> MAGLNEILLPEVHLNSPIVRYKLFYYILHGQLPNDLEPDDLGPLANQNWKAIRAEESQVHARLKQIRVELIARIPSLRWTRSQREIAILIWPRILPILQAYDLRQSMQLPTVWEKLTQSTVNLISDGLERVVLHISNQLTGKPNLFTRSRAGQDTKDYSIPSTRELSQIWFNNEWSGSVKTWLMIKYRMRQLITNQKTGELTDLVTIVDTRSTLCIITPELVALYSSEHKALTYLTFEMVLMVTDMLEGRLNVSSLCTASHYLSPLKKRIEVLLTLVDDLALLMGDKVYGIVSSLESFVYAQLQYGDPVIDIKGTFYGFICNEILDLLTEDNIFTEEEANKVLLDLTSQFDNLSPDLTAELLCIMRLWGHPTLTASQAASKVRESMCAPKVLDFQTIMKTLAFFHAILINGYRRSHNGIWPPTTLHGNAPKSLIEMRHDNSELKYEYVLKNWKSISMLRIHKCFDASPDEDLSIFMKDKAISCPRQDWMGVFRRSLIKQRYRDANRPLPQPFNRRLLLNFLEDDRFDPIKELEYVTSGEYLRDPEFCASYSLKEKEIKATGRIFAKMTKRMRSCQVIAESLLANHAGKLMRENGVVLDQLKLTKSLLTMNQIGIISEHSRRSTADNMTLAHSGSNKHRINNSQFKKNKDNKHEMPDDGFEIAACFLTTDLTKYCLNWRYQVIIPFARTLNSMYGIPHLFEWIHLRLMRSTLYVGDPFNPPSDPTQLDLDTALNDDIFIVSPRGGIEGLCQKLWTMISISTIILSATEANTRVMSMVQGDNQAIAITTRVVRSLSHSEKKEQAYKASKLFFERLRANNHGIGHHLKEQETILSSDFFIYSKRVFYKGRILTQALKNVSKMCLTADILGDCSQASCSNLATTVMRLTENGVEKDLCYFLNAFMTIRQLCYDLVFPQTKSLSQDITNAYLNHPILISRLCLLPSQLGGLNFLSCSRLFNRNIGDPLVSAIADVKRLIKAGCLDIWVLYNILGRRPGKGKWSTLAADPYTLNIDYLVPSTTFLKKHAQYTLMERSVNPMLRGVFSENAAEEEEELAQYLLDREVVMPRVAHVILAQSSCGRRKQIQGYLDSTRTIIRYSLEVRPLSAKKLNTVIEYNLLYLSYNLEIIEKPNIVQPFLNAINVDTCSIDIARSLRKLSWATLLNGRPIEGLETPDPIELVHGCLIIGSDECEHCSSGDDKFTWFFLPKGIRLDDDPASNPPIRVPYIGSKTDERRVASMAYIKGASVSLKSALRLAGVYIWAFGDTEESWQDAYELASTRVNLTLEQLQSLTPLPTSANLVHRLDDGTTQLKFTPASSYAFSSFVHISNDCQILEIDDQVTDSNLIYQQVMITGLALIETWNNPPINFSVYETTLHLHTGSSCCIRPVESCVVNPPLLPVPLINVPQMNKFVYDPEPLSLLEMEKIEDIAYQTRIGGLDQIPLLEKIPLLAHLTAKQMVNSITGLDEATSIMNDAVVQADYTSNWISECCYTYIDSVFVYSGWALLLELSYQMYYLRIQGIQGILDYVYMTLRRIPGMAITGISSTISHPRILRRCINLDVIAPINSPHIASLDYTKLSIDAVMWGTKQVLTNISQGIDYEIVVPSESQLTLSDRVLNLVARKLSLLAIIWANYNYPPKVKGMSPEDKCQALTTHLLQTVEYVEYIQIEKTNIRRMIIEPKLTAYPSNLFYLSRKLLNAIRDSEEGQFLIASYYNSFGYLEPILMESKIFNLSSSESASLTEFDFILNLELSDASLEKYSLPSLLMTAENMDNPFPQPPLHHVLRPLGLSSTSWYKTISVLNYISHMKISDGAHLYLAEGSGASMSLIETFLPGETIWYNSLFNSGENPPQRNFAPLPTQFIESVPYRLIQAGIAAGNGIVQSFYPLWNGNSDITDLSTKTSVEYIIHKVGADTCALVHVDLEGVPGSMNSMLERAQVHALLITVTVLKPGGLLILKASWEPFNRFSFLLTVLWQFFSTIRILRSSYSDPNNHEVYIIATLAVDPTTSSFTTALNRARTLNEQGFSLIPPELVSEYWRKRVEQGQIIQDCIDKVISECVRDQYLADNNIILQAGGTPSTRKWLDLPDYSSFNELQSEMARLITIHLKEVIEILKGQASDHDTLLFTSYNVGPLGKINTILRLIVERILMYTVRNWCILPTQTRLTLRQSIELGEFRLRDVITPMEILKLSPNRKYLKSALNQSTFNHLMGETSDILLNRAYQKRIWKAIGCVIYCFGLLTPDVEGSERIDVDNDIPDYDIHGDII;>MDQFIKQDETGDLIETGMNVANHFLSTPIQGTNSLSKASILPGVAPVLIGNPEQKNIQHPTASHQGSKTKGRGSGVRSIIVSPSEAGNGGTQIPEPLFAQTGQGGIVTTVYQDPTIQPTGSYRSVELAKIGKERMINRFVEKPRTSTPVTEFKRGGPGAAAQGQTIQEEGIDGNGASAGSKERSGSLSGATLYAHLSLPQQDSTPANVGIAPQSAISANEIMDLLRGMDARLQHLEQKVDKVLAQGSMVTQIKNELSTVKTTLATIEGMMATVKIMDPGNPTGVPVDELRRSFSDHVTIVSGPGDVSFSSSEKPTLYLDELARPVSKPRPAKQTKSQPVKDLAGQKVMITKMITDCVANPQMKQAFEQRLAKASTEDALNDIKRDIIRSAI[4x]

L and P function as the RNA polymerase complex, responsible for replicating and transcribing the viral genome. To catalyze the RNA synthesis in both replication and transcription, L sequentially consists of five domains: the RNA-dependent RNA polymerase domain (RdRp), polyribonucleotidyl transferase domain (PRNTase), connector domain (CD), methyltransferase domain (MTase), and C-terminal domain (CTD). P harbors an oligomerization domain (POD) for self-oligomerization, and the oligomeric P attaches to RdRp of L, tethering the polymerase to NC to extract the RNA strand for both replication and transcription. Here, we resolved two L–P complex conformations from the mumps virus (MuV), a typical member of nsNSVs, via cryogenic-electron microscopy.

The other conformation has CD-MTase-CTD averaged out due to the structural flexibility, with its RNA tunnel inaccessible to MTase, unfavorable for genome transcription. Following the same strategy, Lbody–P was determined at the resolution of 3.01 Å, and only RdRp and PRNTase are visible in L. The missing of appendage in Lbody–P indicates the structural flexibility in MuV L–P, as in other nsNSVs. MuV Lbody–P owns a flexible appendage, and its RNA tunnel is inaccessible to MTase-CTD, which is unfavorable for transcription. However, the RNA cavity formed by RdRp and PRNTase domains is available, with the potential capability for genome replication. MuV Lbody–P takes an appendage-free conformation but still owns an exposed RNA cavity formed by RdRp and PRNTase domains with the potential to another replication state for RNA synthesis. Models in (c, e) are the composite atomic models of MuV Lintegral–P and Lbody–P via rigid body docking of individual models into their respective composite cryo-EM maps, which are B-factor sharpened. In both conformations, parallel P tetramers are revealed around MuV L, which, together with structures of other nsNSVs, demonstrates the diverse origins of the L-binding X domain of P. Our study links varying structures of nsNSV polymerase complexes with genome replication and transcription and points to a sliding model for polymerase complexes to advance along the RNA templates.>[2x]GSNFCDSKCKL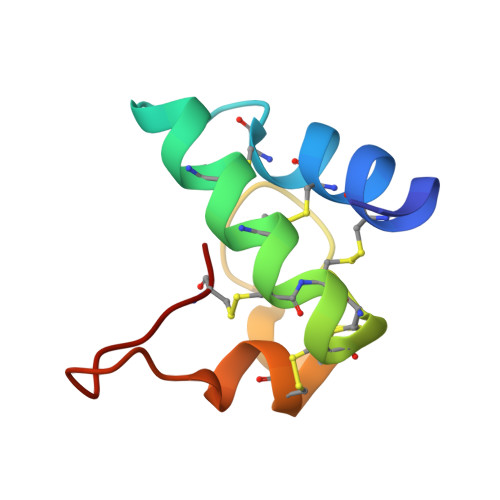RCSKAGLADRCLKYCGICCEECKCVPSGTYGNKHECPCYRDKKNSKGKSKCP>MHHHHHHENLYFQGNGITLPDFEQDFNHIKGGFAPMFNNIQVLTPEWVYQLQQGLNSDIWSGYMATPTGFESGVNNTTYALLDNWNGFIWDYGYKNVMFNAYDIANKSKGKYDQFYALSLILKVEGMHRMTDTFGPIIYSKFGSNDATIAYDSQEEVYTQMFAE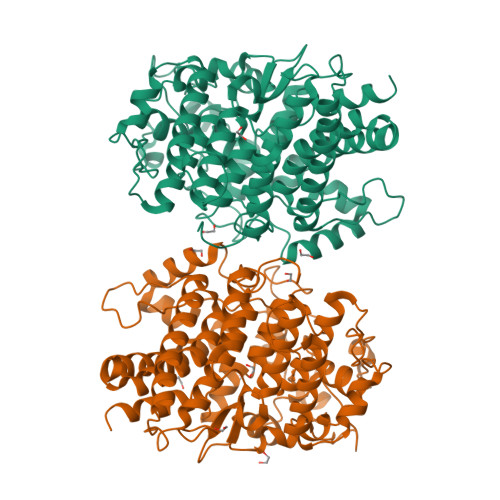LDTAVAELTKRIDAGEASTFESTDMTGYKGKYESWVRFANTLRLRLAMRIVKVKPALAKTEAEKAVAQKFGVMLVNDDSFKIVSPVYTNPIATISSSWLDIRMSADMESIMKGYQDPRIASYFDTSKQFPNEYKGVRTGIAISGKSDHQDFSGIGAVVRSKEIYLMNAAEAYFLRAEGALRGWNMGGTAQELYEAGIKASFDQRGVSGAAGYIADNTKTAAAYVDPNFPENNSDPVNNVTVAWDAAATNEVKLQKIITQKWIAGFPEGQEAWSDYRRTGYPKLFPVLKNYSGGAITTEFGVRRINFVQSEKAGNSGGVATGVSKLGGPDNGGTRVWWDVNAPNF[2x]>[4x]VPALTREQLYIFDTTGFLVIPGVFGSGEVESFRSELERLDTVDPGFPRTRRYPDLPAASPVFARLALDDRLLAPVRDVVNQPLRLLEGYGLRRTKDSVLYLHGGNSELLDLGDRQVGRDLSITHTYHDGKLYCPYVKALVYLSDIQSPEDGSFCYVQGSHKAN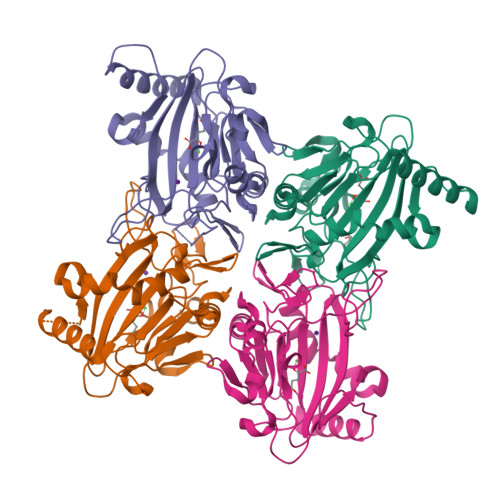FPLLRERAERGENTSLVDSGFPTLSDVFVRSGDVLLLNEALMHGTRRKLTEGDRLLTAFGYGPTFFTEWRELDAETADLRGAGYVDHDVEEDFVL>[2x]MEFNLHAVSSEEKERDFDVVIVGAGAAGFSAAVYAARSGFSVAILDKAVAGGLTAEAPLVENYLGFKSIVGSELAKLFADHAANYAKIREGVEV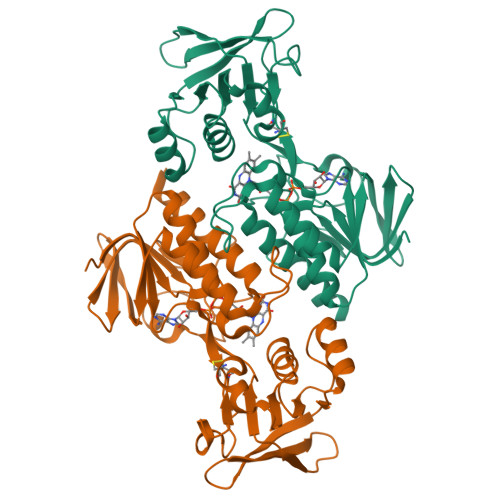RSIKKTQGGFDIETNDDTYHAKYVIITTGTTHKHLGVKGESEYFGKGTSYCSTCDGYLFKGKRVVTIGGGNSGAIAAISMSEYVKNVTIIEYMPKYMCENAYVQEIKKRNIPYIMNAQVTEIVGDGKKVTGVKYKDRTTGEEKLIETDGVFIYVGLIPQTSFLKDSGVKLDERGYIVVDSRQRTSVPGVYAAGDVTSGNFAQIASAVGDGCKAALSLYSDSISKK S-(2-acetamidoethyl) (2S)-2-azanyl-4-methyl-pentanethioate 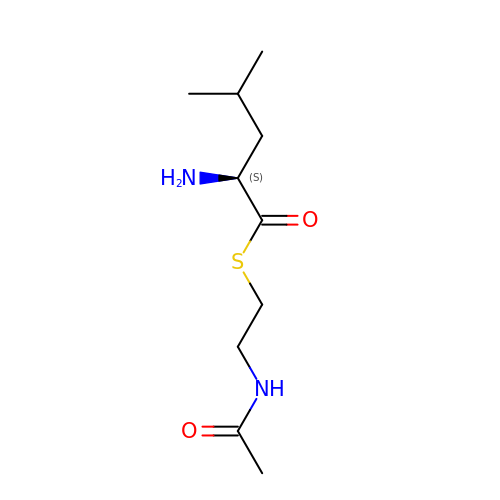| C10 H20 N2 O2 S | FGUKBCKKFXHYHQ-VIFPVBQESA-N>[3x]MDTRTRHLKVSNCPNNSYALANVAAVSPNDFPNNIYIII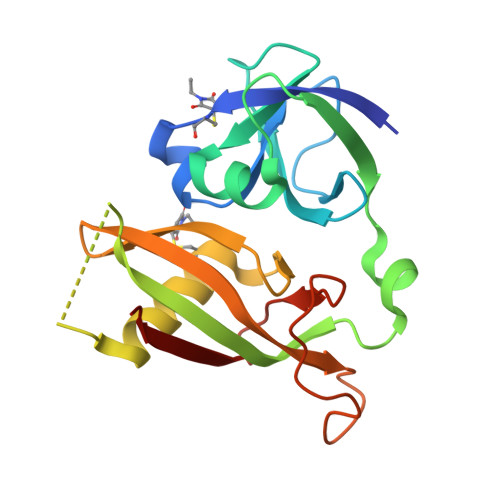DNLFVFTTRHSNDIPPGTIGFNGNQRTWGGWSLNQDVQAKAFDLFKYSGKQSYLGSIDIDISFRARGKAVSTVFDQDELAKQFVRCYESQIFSPTQYLIMEFQGHFFDLKIRNVQAIDLGDIEPTSAVATGIETKGILTKQTQINFFKGR> SPDKQMAVLPRRERNRQAAAANPENSRGKGRRGQRGKNRGCVLTAIHLNVTD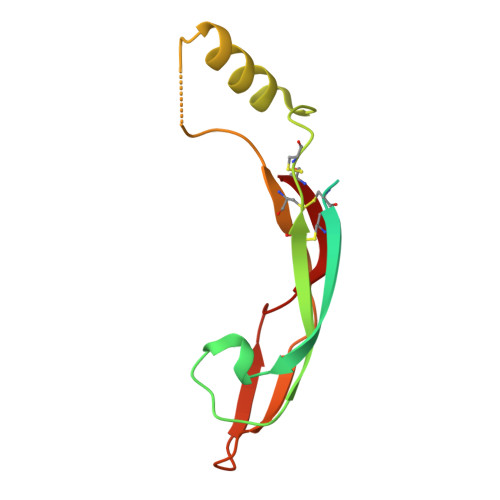LGLGYETKEELIFRYCSGSCDAAETTYDKILKNLSRNRRLVSDKVGQACCRPIAFDDDLSFLDDNLVYHILRKHSAKRCGCI> SNAFHPVYSVQLEQKLVEKFNLKRALISLDQPNTNEQRKQVAALVSSYLNNNLQEGMAVAVGQGQNVAAVADHAGIVTQRNARFVSAIGGTHRSGDIINADHICRRLAKKYGGSSETLYAPAYVNDPSLR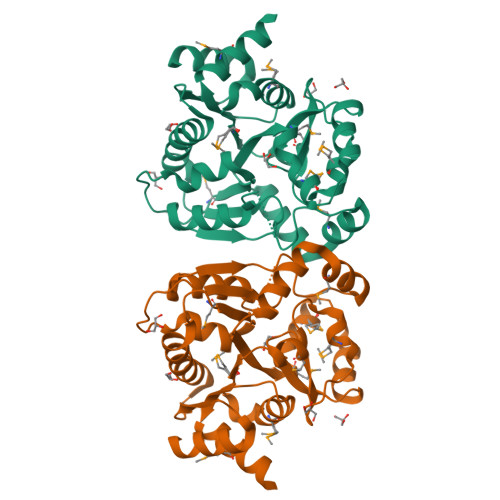SAFMEHATIKETLSQARKAEFALVGIGDMDENSHMVKLGFFTPKEFVEARLNDGIVGDIGGFDFFKLDGTDADTLMRGRVIGLEMEDLRQIPNVVAMASESRKALSIMGALRTGVIDVLATSVSCAMALLNLAENEE>[2x]HHHHHHSSGHIDDDDKMAPSILSTESSIIVIGAGTWGCSTALHLARRGYKDVTVLDPHPVPSPIAAGNDINKIMEHSELKDGCSDPRSAAFSTFTRAALKAWKTDPVFQPYFHETGFIISGHT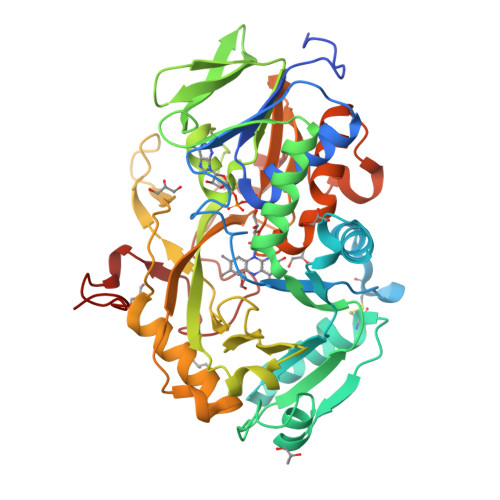PALIDHIRKDEVECSETNFVKLETAEDFRRTMPPGVLTGDFPGWKGWLHKSGAGWIHAKKAMISAFNEAKRLGVRFVTGSPEGNVVSLVYEDGDVVGARTADGRVHKAHRTILSAGAGSDSLLDFKKQLRPTAWTLCHIQMGPEEVKQYRNLPVLFNIAKGFFMEPDEDKHELKICDEHPGYCNFLPDPNRPGQEKSVPFAKHQIPLEAEARARDFLHDTMPHLADRPLSFARICWDADTPDRAFLIDRHPEHPSLLVAVGGSGNGAMQMPTIGGFIADALESKLQKEVKDIVRWRPETAVDRDWRATQNRFGGPDRIMDFQQVGEDQWTKIGESRGP>GSHMTEEEVRKIMEKLKKAFKQGNPEQIVSLLSPDVKVDVGNQSFSGSEEAEKAARKLMKFVDRVEVRDVRVFENAVMIAVEFEVNGQRYKMIFTFYVENGKVSMVSIYISPTMKKLMKQILNYG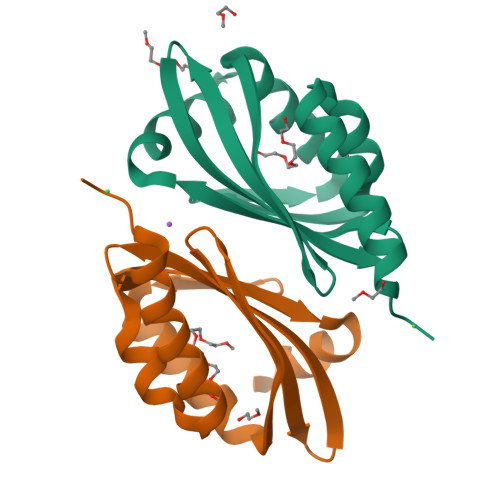[2x]>ASMTGGQQMGRGSASLPACPEESPLLVGPMLIEFNMPVDLELVAKQNPNVKMGGRYAPRDCVSPHKVAIIIPFRNRQEHLKYWLYYLHPVLQRQQLDYGIYVINQAGDTIFNRAKLLNVGFQEALKDYDYTCFVFSDVDLIPMNDHNAYRCFSQPRHISVAMDKF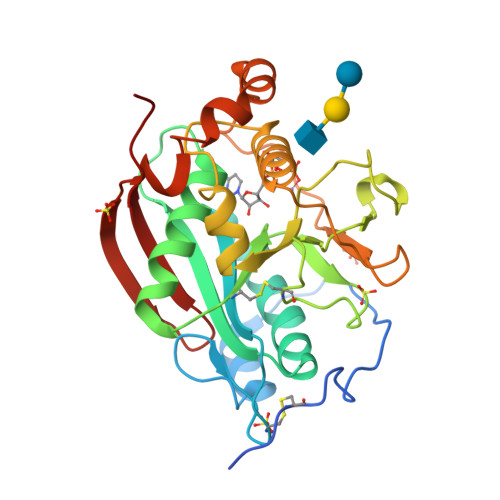GFSLPYVQYFGGVSALSKQQFLTINGFPNNYWGWGGEDDDIFNRLVFRGMSISRPNAVVGTTRHIRHSRDKKNEPNPQRFDRIAHTKETMLSDGLNSLTYQVLDVQRYPLYTQITVDIGTPS[3x]>MIVPVLSRQALRHASVARVALPSLTRWYASYPPHTVVKMPALSPTMTSGGIGAWQKKPGDKIEPGEVLVEIETDKAQMDFEFQEEGVLAKILKDSGEKDVAVGNPIAILVEEGTDVNAFKDFTLKDAGGETSPAVPKDEPKNESTASAPTPAPTPAPEPENTSFTGRFQTALEREPNALPAAKRLAREKGIDLRNVKGSGPGGKITEEDVKKALASAPAAGAAAAAYTDVPISGMRKTIAARLKESVTENPHFFVSTNLSVSKLLKLRQAL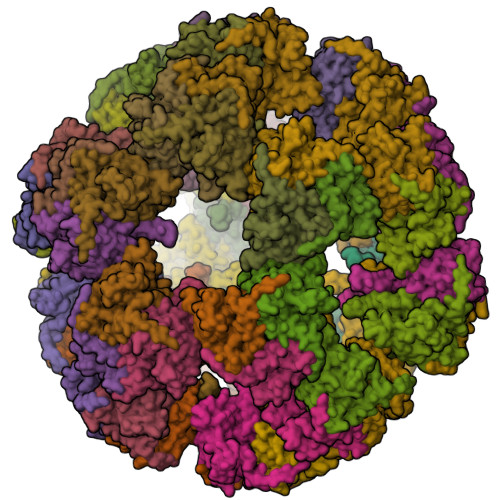NSSADGRYKLSVNDFLIKAMGIASKRVPTVNSSWRDGVIRQFETVDVSVAVATPNGLITPIVKGVEGKGLESISAAVKELAKKARDGKLKPEEYQGGSISISNMGMNPAVQSFTAIINPPQAAILAVGAPQKVAVPVENEDGTTGVSWDEQIIVTASFDHKVVDGAVGAEWIRELKKVIENPLELLL[60x]> MAITAKPKAGVWAVLWDLLTTVDHKKIGLMYTATAFFAFALAGVFSLLIRTQLAVPNNQFLTGEQYNQILTLHGATMLFFFIIQAGLTGFGNFVVPLMLGARDVALPRVNAFSYWAFLGAIVLALMSYFFPGGAPSVGWTFYYPFSAQSESGVDFYLAAILLLGFSSLLGNANFVATIYNLRAQGMSLWKMPIYVWSVFAASVLNLFSLAGLTAATLLVLLERKIGLSWFNPAVGGDPVLFQQFFWFYSHPTVYVMLLPYLGILAEVASTFARKPLFGYRQMVWAQMGIVVLGTMVWAHHMFTVGESTL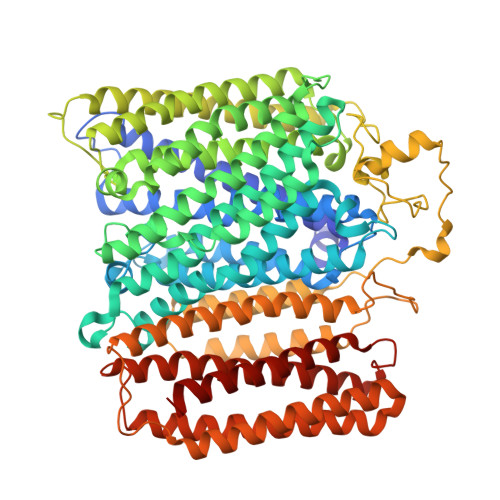FQIAFAFFTALIAVPTGVKLFNIIGTLWGGKLQMKTPLYWVLGFIFNFLLGGITGVMLSMTPLDYQFHDSYFVVAHFHNVLMAGSGFGAFAGLYYWWPKMTGRMYDERLGRLHFWLFLVGYLLTFLPQYALGYLGMPRRYYTYNADIAGWPELNLLSTIGAYILGLGGLVWIYTMWKSLRSGPKAPDNPWGGYTLEWLTASPPKAHNFDVKLPTEFPSERPLYDWKKKGVELKPEDPAHIHLPNSSFWPFYSAATLFAFFVAVAALPVPNVWMWVFLALFAYGLVRWALEDEYSHPVEHHTVTGKSNAWMGMAWFIVSEVGLFAILIAGYLYLRLSGAATPPEERPALWLALLNTFLLVSSSFTVHFAHHDLRRGRFNPFRFGLLVTIILGVLFFLVQSWEFYQFYHHSSWQENLWTAAFFTIVGLHGLHVVIGGFGLILAYLQALRGKITLHNHGTLEAASMYWHLVDAVWLVIVTIFYVW>TSSANEDMPVERILEAELAVEPKTETYVEANMGLNPSSPNDPVTNICQAADKQLFTLVEWAKRIPHFSELPLDDQVILLRAGWNELLIASFSHRSIAVKDGILLATGLHVHRNSAHSAGVGAIFDRVLTELVSKMRDMQMDKTELGCLRAIVLFNPDSKGLSNPAEVEALREKVYASLEAYCKHKYPEQPGRFAKLLLRLPALRSIGLKCLEHLFFFKLIGDTPIDTFLMEMLEAPHQMT[2x];>HKILHRLLQD[2x]

Nuclear receptors are ligand-regulated transcription factors, involving multiple signalling pathways, among which RXRα and PPARγ are in the central positions. Once activated by their agonists, RXRα and PPARγ translocate into the nucleus forming RXRα:RXRα homodimer or RXRα:PPARγ heterodimer, which subsequently binds to RXRE or PPRE to initial their target genes transcription, respectively. Interestingly, we find that magnolol is a dual agonist of both RXRα and PPARγ. To reveal the molecular basis for magnolol function, we determine the crystal structures of both RXRαLBD-magnolol and PPARγLBD-magnolol.

RXRα plays its role in diverse physiological processes, including cell development, apoptosis, and homeostasis. As indicated in the previously reported crystal structures of RXRα ligand-binding domain complex with agonists, the essential activation function-2 (AF-2) motif in RXRα exhibits significant conformational changes. AF-2 motif overturns itself to cover the ligand-binding pocket upon agonist binding, thus exposing the surface for recruiting the coactivator SRC1 and initializing the transcription of target genes. The typical chemical structure of RXRα agonist consists of the acidic and hydrophobic moieties to adapt the L-shaped ligand-binding pocket of RXRα. Different from previously reported RXRα agonists, magnolol possesses two identical 5-allyl-2-hydroxyphenyl moieties. To reveal the molecular basis for magnolol binding and activating RXRα, we determine the crystal structure of RXRαLBD-magnolol complex with SRC1 coactivator peptide. Magnolol-bound RXRαLBD exhibits a dimeric packing of RXRα. In RXRαLBD-magnolol structure, the hydroxyl group of magnolol contacts with Asn306 in helix 5 of RXRα. Although magnolol is big enough to accommodate mostly the L-shaped RXRα ligand-binding pocket, two magnolol molecules have to cooperatively occupy the much larger Y-shaped PPARγ ligand-binding pocket. Furthermore, the single bond connecting the two 5-allyl-2-hydroxyphenyl moieties of magnolol endows this chemical compound flexibility to fit the different pocket sizes of RXRα and PPARγ.> SNAMGFLILS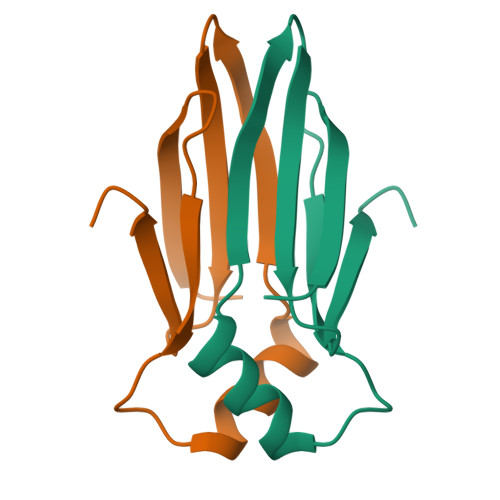RREGEGITLSLKADYPAEELIRQLREGGIRILVTDIIGNQARVGIEAPRGVLIVRDELKTAPKG>MNQKHSSDFVVIKAVEDGVNVIGLTRGTDTKFHHSEKLDKGEVIIAQFTEHTSAIKVRGEALIQTAYG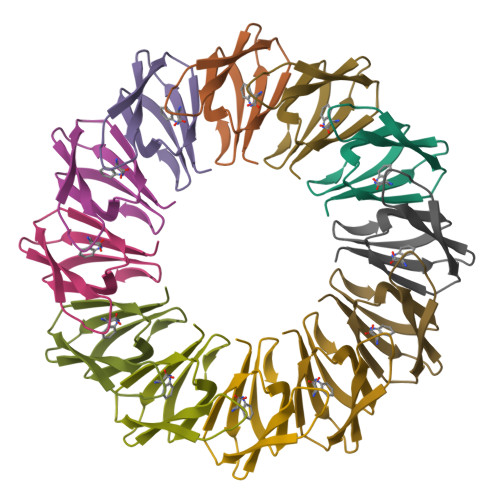EMKNEKK[6x]>[2x]PTSLKDTVKLHNGVEMPWFGLGVFKVENGNEATESVKAAIKNGYRSIDTAAIYKNEEGVGIGIKESGVAREELFITSKVWNEDQGYETTLAAFEKSLERLQLDYLDLYLIHWPGKDKYKDTWRALEKLYKDGKIRAIGVSNFQVHHL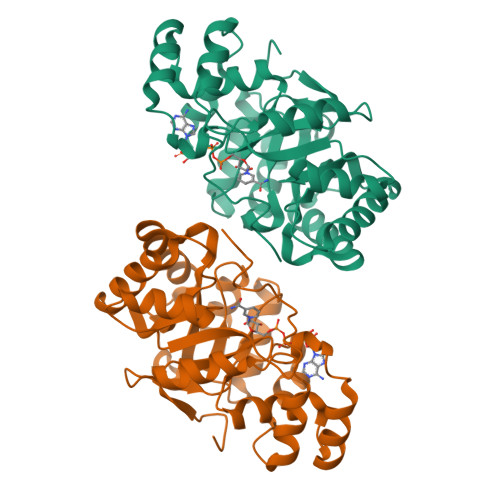EELLKDAEIKPMVNQVEFHPRLTQKELRDYCKGQGIQLEAWSPLMQGQLLDNEVLTQIAEKHNKSVAQVILRWDLQHGVVTIPKSIKEHRIIENADIFDFELSQEDMDKIDALNKDERVGPNPDELLF>SMRWKRMMQLLDVHCEGEIGKVAIGGVPKIPGDTVADQLHWLNTDPKGRELRHFLVLEPRGAPIGSVNLLLPAKDSRADAAFIILQPDQAHASSGSNSICVTTALLESGMIEMQEPETVVMLETAAGLVKAVAQCRDGHCDSVTLTMVPSFVHELDAQIATESWGEIRFDLAYGGVFYALVDVRQLGLTIEPGNARRLVEAGMLLKGEINQRIQVVHPDIPAISGVAYVMFRDEDPDGAVRTCTTMWPGRVDRSPCGTGNSANLATLHARGRVKPGDSFLSRSIIGSQFTVGLQGLT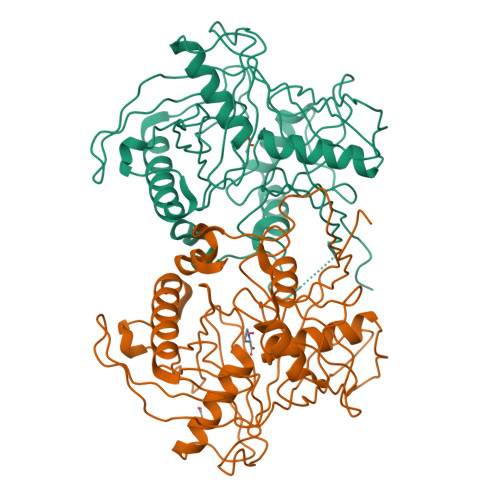TVAGRSAVIPTITGRGFTYGIHQVALDAFDPLGGGFVLTDVWGAAAETIKI[2x]Unlike other PLs, Smlt1473 present in the clinically relevant Stenotrophomonas maltophilia strain K279a demonstrates a wide range of pH-dependent substrate specificities toward multiple, diverse polysaccharides: hyaluronic acid (pH 5.0), poly-β-D-glucuronic (celluronic) acid (pH 7.0), poly-β-D-mannuronic acid, and poly-α-L-guluronate (pH 9.0). To decode the pH-driven multiple substrate specificities and selectivity in this single enzyme, we present the X-ray structures of Smlt1473 determined at multiple pH values in apo and mannuronate-bound states as well as the tetra-hyaluronate-docked structure. We have built and refined the structures from residues A22-L330; electron density for other residues outside this range was either weak or absent. The structure is composed of 13 α-helical segments (α-1 to α-13) connected by 14 loops (L-1 to L-14) and two β-strands (β-1 and β-2) (Fig. 2, B and C (i and ii)).

We used the tetra unit of HA [NAG (+2) (3←1) BDP (+1) (4←1) NAG (−1) (3←1) BDP (−2)] for cocrystallization with inactive mutant H168A at pH 5.0. After solving the structure, we found a significant region of diffuse electron density within the active site, but we did not observe any specific, resolvable interactions with water or other solutes. Furthermore, we were unable to model an individual sugar unit within the region of diffuse electron density, as it was not large enough to accommodate a pyranose ring including its substituents. Since we know the specific region within the tunnel that corresponds to polysaccharide binding from our high-resolution ManA-complexed enzyme structures, we performed docking studies for tetra unit of HA by taking the protein coordinates of wild-type Smlt1473 bound to tetra-ManA at pH 5. Specifically, we used the Rosetta flexible ligand protocol to generate a large number of possible models, and by utilizing scoring parameters we were able to find the most plausible tetra-HA-docked structure.

> ACPAPPPGQPDIRAIGYYTDKAGSVIDPALQQQNKDATAPLDRYAADVARMSDDYLRNGDPAAAQCTLSWLGAWADDGAMLGQMIRVNNDQSFYMRQWMLDAVAMAYLKVHDQANPQQRARIDPWLQKLARANLAYWDNPKRRRNNAYYWGGLGVLATGLATDDDALWQAGHAAFQKGIDDIQDDGSLPLEMARGQRALHYHDYALAPLVMMAELARLRGQDWYASRNHAIDRLARRVIEGSRDPAWFNQHTGAAQLPLQASGWVEFYRLRSPDGGVFDAAHARGPFHSPRLGGDLTLMATHGIVRTPLRHHHHHH> GSGGIEGRHMELMGKLDKASKLIDEENKYYARSARINYYNLVIDHAHGATLVDVDGNKYIDLLASASAINVGHTHEKVVKAIADQAQKLIHYTPAYFHHVPGMELSEKLAKIAPGNSPKMVSFGNSGSDANDAIIKFARAYTGRQYIVSYMGSYHGSTYGSQTLSGSSLNMTRKIGPMLPSVVHVPYPDSYRTYPGETEHDVSLRYFNEFKKPFESFLPADETACVLIEPIQGDGGIIKAPEEYMQLVYKFCHEHGILFAIDEVNQGLGRTGKMWAIQQFKDI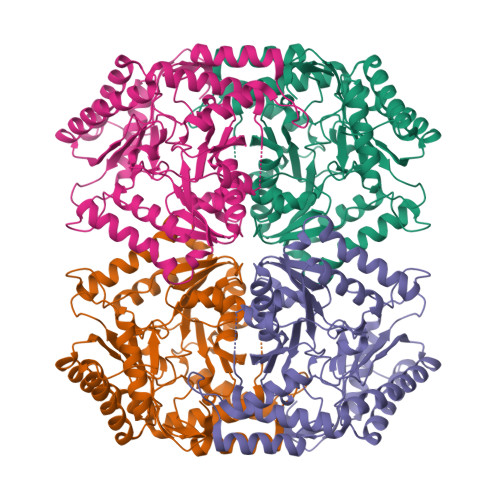EPDLMSVGKSLASGMPLSAVIGKKEVMQSLDAPAHLFTTAGNPVCSAASLATLDVIEYEGLVEKSATDGAYAKQRFLEMQQRHPMIGDVRMWGLNGGIELVKDPKTKEPDSDAATKVIYYAFAHGVVIITLAGNILRFQPPLVIPREQLDQALQVLDDAFTAVENGEVTIPKDTGKIGW> MQASQFSAQVLDWYDKYGRKTLPWQIDKTPYKVWLSEVMLQQTQVATVIPYFERFMARFPTVTDLANAPLDEVLHLWTGLGYY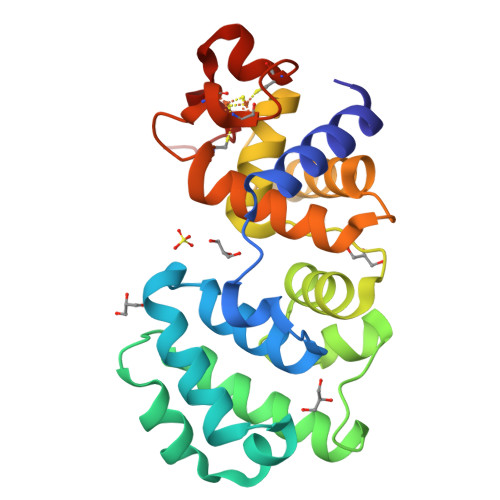ARARNLHKAAQQVATLHGGKFPETFEEVAALPGVGRSTAGAILSLSLGKHFPILDGNVQRVLARCYAVSGWPGKKEVENKLWSLSEQVTPAVGVERFNQAMMDLGAMICTRSKPKCSLCPLQNGCIAAANNSWALYPGKKPK>QLNPYLRLKVRRDHIIDDALVRLEMIAMENPADLKKQLYVEFEGEQGVDEGGVSKEFFQLVVEEIFNPDIGMFTYDESTKLFWFNPSSFETEGQFTLIGIVLGLAIYNNCILDVHFPMVVYRKLMGKKGTFRDLGDSHPVLYQSLKDLLEYEGNV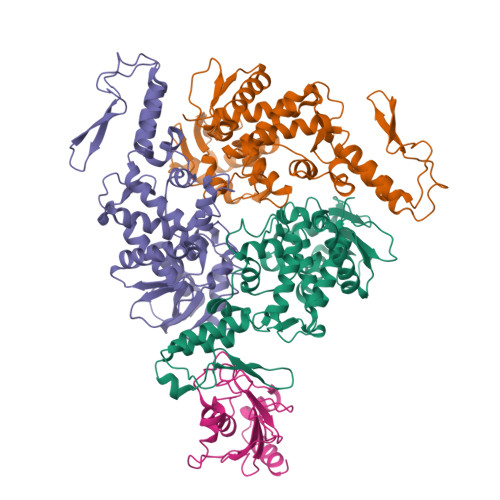EDDMMITFQISQTDLFGNPMMYDLKENGDKIPITNENRKEFVNLYSDYILNKSVEKQFKAFRRGFHMVTNESPLKYLFRPEEIELLICGSRNLDFQALEETTEYDGGYTRDSVLIREFWEIVHSFTDEQKRLFLQFTTGTDRAPVGGLGKLKMIIAKNGPDTERLPTSHTCFNVLLLPEYSSKEKLKERLLKAITYAKGFGML[3x];> MAASRRLMKELEEIRKCGMKNFRNIQVDEANLLTWQGLIVPDNPPYDKGAFRIEINFPAEYPFKPPKITFKTKIYHPNIDEKGQVCLPVISAENWKPATKTDQVIQSLIALVNDPQPEHPLRADLAEEYSKDRKKFCKNAEEFTKKYGEKRPVD>GSHMSGTEEAILGGRDSHPAAGGGSVLCFGQCQYTAEEYQAIQKALRQRLGPEYISSRMAGGGQKVCYIEGHRVINLANEMFGYNGWAHSITQQNVDFVDLNNGKFYVGVCAFVRVQLKDGSYHEDVGYGVSEGLKSKALSLEKARKEAVTDGLKRALRSFG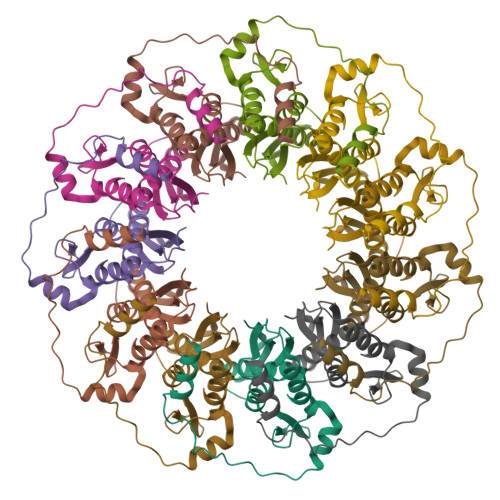NALGNCILDKDYLRSLNKLPRQLPLEVDLTKAKRQDLEPSVEEARYNSCRPNMALGHPQLQQVTSPSRPSHAVIPADQDCSSRSLSSSAVESEATHQRKLRQKQLQQQFRERMEKQQVRVSTPSAEKSEAAPPAPPVTHSTPVTVSEPLLEKDFLAGVTQELIKTLEDNSEKWAVTPDAGDGVVKPSSRADPAQTSDTLALNNQMVTQNRTPHSVCHQKPQAKSGSWDLQTYSADQRTTGNWESHRKSQDMKKRKYDPS[11x]>GSSVTVRPDWVTIEEMDFPRLSKLTLPGVKEGEDVLCCGAVEYYDKSYD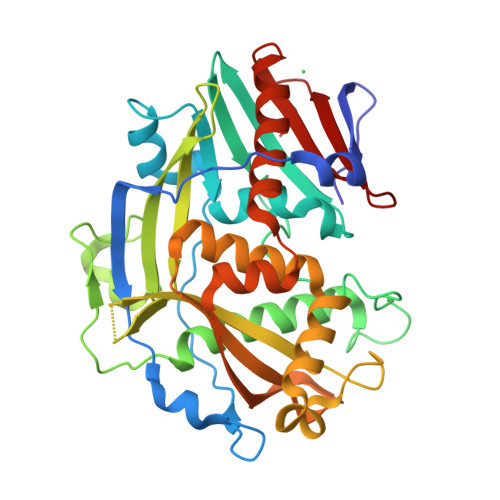RVNVKNEKPLQRIDRIFHTVTTTDDPVIRKLSKTEGNVYATDAILATIMCCTRSNYSWDIVIEKIGNKLFFDKRDNTEFDLLTVNETSVEPPQDDGNSLNSPRNLALEATFINHNFSQQVLKSNEPRYKFDEPNPFISEEEEGEVASVAYRYRKWDLNNGITLIARCEHDAVMQGPNNETQFLTIKALNEWDSKLANGVEWRRKLDTQRGAVLANELRNNACKLAKWTVQALLAGSDQLKFGYVSRASVRDSSKHVILETQQYKPNEFATQINLNMDNAWGILRCIIDICMNQKDGKYLIMKDPNKPMIRLYDIPDNTF[2x]> MDEIISELRELCLNYIEQDERLSRQKLNFLGQREPRMVLIEGLKLLSRCIEIDSADKSGCTHNHDDKSVETILVESGIVCPGLPLIIPDGYKLIDNSLILLECFVRSTPASFEKKFIEDTNKLACIREDLAVAGVTLVPIVDGRCDYDNSFMPEWANFKFRDLLFKLLEYSNQNEKVFEESEYFRLCESLKTTIDKRSGMDSMKILKDARSTHNDEIMRMCHEGINPNMSCDDVVFGINSLFSRFRRDLESGKLKRNFQKVNPEGLIKEFSELYENLADSDDILTLSREAVESCPLMRFITAETHGHERGSETSTEYERLLSMLNKVKSLKLLNTRRRQLLNLDVLCLSSLIKQSKFKGLKNDKHWVGCCYSSVNDRLVSFHSTKEEFIRLLRNRKKSKVFRKVSFEELFRASISEFIAKIQKCLLVVGLSFEHYGLSEHLEQECHIPFTEFENFMKIGAHPIMYYTKFEDYNFQPSTEQLKNIQSLRRLSSVCLALTNSMKTSSVARLRQNQIGSVRYQVVECKEVFCQVIKLDSEEYHLLYQKTGESSRCYSIQGPDGHLISFYADPKRFFLPIFSDEVLYNMIDIMISWIRSCPDLKDCLTDIEVALRTLLLLMLTNPTKRNQKQVQSVRYLVMAIVSDFSSTSLMDKLREDLITPAEKVVYKLLRFLIKTIFGTGEKVLLSAKFKFMLNVSYLCHLITKETPDRLTDQIKCFEKFFEPKSQFGFFVNPKEAITPEEECVFYEQMKRFTSKEIDCQHTTPGVNLEAFSLMVSSFNNGTLIFKGEKKLNSLDPMTNSGCATALDLASNKSVVVNKHLNGERLLEYDFNKLLVSAVSQITESFVRKQKYKLSHSDYEYKVSKLVSRLVIGSKGEETGRSEDNLAEICFDGEEETSFFKSLEEKVNTTIARYRRGRRANDKGDGEKLTNTKGLHHLQLILTGKMAHLRKVILSEISFHLVEDFDPSCLTNDDMKFICEAVEGSTELSPLYFTSVIKDQCGLDEMAKNLCRKFFSENDWFSCMKMILLQMNANAYSGKYRHMQRQGLNFKFDWDKLEEDVRISERESNSESLSKALSLTKCMSAALKNLCFYSEESPTSYTSVGPDSGRLKFALSYKEQVGGNRELYIGDLRTKMFTRLIEDYFESFSSFFSGSCLNNDKEFENAILSMTINVREGFLNYSMDHSKWGPMMCPFLFLMFLQNLKLGDDQYVRSGKDHVSTLLTWHMHKLVEVPFPVVNAMMKSYVKSKLKLLRGSETTVTERIFRQYFEMGIVPSHISSLIDMGQGILHNASDFYGLLSERFINYCIGVIFGERPEAYTSSDDQITLFDRRLSDLVVSDPEEVLVLLEFQSHLSGLLNKFISPKSVAGRFAAEFKSRFYVWGEEVPLLTKFVSAALHNVKCKEPHQLCETIDTIADQAIANGVPVSLVNSIQRRTLDLLKYANFPLDPFLLNTNTDVKDWLDGSRGYRIQRLIEELCPNETKVVRKLVRKLHHKLKNGEFNEEFFLDLFNRDKKEAILQLGDLLGLEEDLNQLADVNWLNLNEMFPLRMVLRQKVVYPSVMTFQEERIPSLIKTLQNKLCSKFTRGAQKLLSEAINKSAFQSCISSGFIGLCKTLGSRCVRNKNRENLYIKKLLEDLTTDDHVTRVCNRDGITLYICDKQSHPEAHRDHICLLRPLLWDYICISLSNSFELGVWVLAEPTKGKNNSENLTLKHLNPCDYVARKPESSRLLEDKVNLNQVIQSVRRLYPKIFEDQLLPFMSDMSSKNMRWSPRIKFLDLCVLIDINSESLSLISHVVKWKRDEHYTVLFSDLANSHQRSDSSLVDEFVVSTRDVCKNFLKQVYFESFVREFVATTRTLGNFSWFPHKEMMPSEDGAEALGPFQSFVSKVVNKNVERPMFRNDLQFGFGWFSYRMGDVVCNAAMLIRQGLTNPKAFKSLKDLWDYMLNYTKGVLEFSISVDFTHNQNNTDCLRKFSLIFLVRCQLQNPGVAELLSCSHLFKGEIDRRMLDECLHLLRTDSVFKVNDGVFDIRSEEFEDYMEDPLILGDSLELELLGSKRILDGIRSIDFERVGPEWEPVPLTVKMGALFEGRNLVQNIIVKLETKDMKVFLAGLEGYEKISDVLGNLFLHRFRTGEHLLGSEISVILQELCIDRSILLIPLSLLPDWFAFKDCRLCFSKSRSTLMYETVGGRFRLKGRSCDDWLGGSVAEDID

Lymphocytic choriomeningitis virus (LCMV) is the prototypic member of the Arenaviridae family and belongs to the Old World (OW) arenavirus together with Lassa virus (LASV), which are distinct from the New World (NW) arenavirus [e.g. Machupo virus (MACV) and Junin virus (JUNV)]. As a segmented negative-sense single-stranded RNA virus (sNSRV), arenavirus encodes a large polymerase (L) to form a ribonucleoprotein complex (RNP) together with the genomic-length RNA encapsidated by viral nucleoprotein (NP) and facilitate virus replication and transcription. Arenavirus also encodes a RING finger Z matrix protein as a regulator of RNA synthesis. Previous studies have shown that the arenavirus Z protein forms a species-specific complex with the L protein and inhibits RNA synthesis initiation by impairing the catalytic activity of the L protein, which is known to be essential for the balance of infection and further initiation of virion assembly; however, the mechanism remains unclear.

After motion correction, contrast transfer function (CTF) estimation, iterative rounds of 2D classification, and heterogeneous 3D refinement, a total of 405,657 particles remained in two classes representing the individual L and the L–Z complex, respectively. Homogeneous 3D refinement of these two particle stacks resulted in a 3.4-Å map for the individual L protein and a 3.6-Å map for the L–Z complex. LCMV-L displays a similar architecture to LASV and MACV-L proteins, with r.m.s.d of 1.882 and 2.729 for 1,282 and 1,110 aligned Cα atoms, respectively, which is consistent with their relatively high amino acid similarities. According to the structures of LASV/MACV-L, the polypeptide of LCMV-L can be divided into three parts: the N-terminal PA-like region, the RdRp region (PB1-like domain), and the C-terminal PB2-like region. We assigned residues to LCMV-L domains as follows: residues 1–190 belong to the endonuclease (endoN) domain; a linker region spans residues 200–259; residues 260–705 belong to a PA-C-like domain; residues 706–1,600 belong to the RdRp core; residues 1,601–1,814 belong to a PB2-like domain, in which residues 1,601–1,727 and 1,799–1,814 belong to the Thumbing ring domain; and residues 1,728–1,798 are a lid domain. The RdRp region is caught in the middle by the PA-like domain, where the PA-C-like region tightly binds to the Thumb domain of the RdRp region and the endoN domain is on the other side. The C-terminal residues 1,815–2,210 cannot be observed in the cryo-EM densities of LCMV-L and the L–Z complex, which is similar to that observed in monomeric LASV/MACV-L and L–Z. This portion is supposed to adopt the cap-binding domain that may have a flexible architecture, as observed in influenza virus polymerase.> YVSESEPLVRFKNSVKITKGDLNSWREGTDPCSGKWFGIYCQKGLTVSGIHVTRLGLSGTITVDDLKDLPNLKTIRLDNNLLSGPLPHFFKLRGLKSLMLSNNSFSGEIRDDFFKDMSKLKRLFLDHNKFEGSIPSSITQLPQLEELHMQSNNLTGEIPPEFGSMKNLKVLDLSTNSLDGIVPQSIADKKNLAVNLTENEYLCGPVVDVGCENIELNDPQ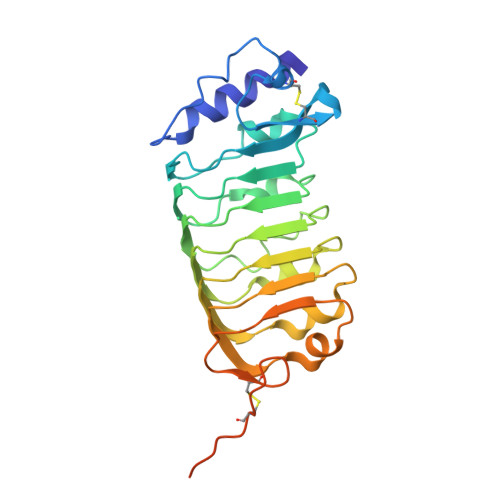EGQPPSKPSSSVPETSHHHHHH4-S-GLUTATHIONYL-5-PENTYL-TETRAHYDRO-FURAN-2-OL | C19 H33 N3 O8 S | 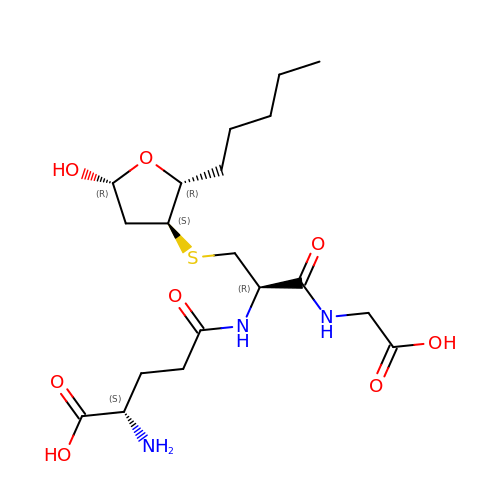ICRIFHIWWXQBPY-JEJJNBGPSA-N> EAIKKLVGLQAKTAVVIRDGKEIAVPVE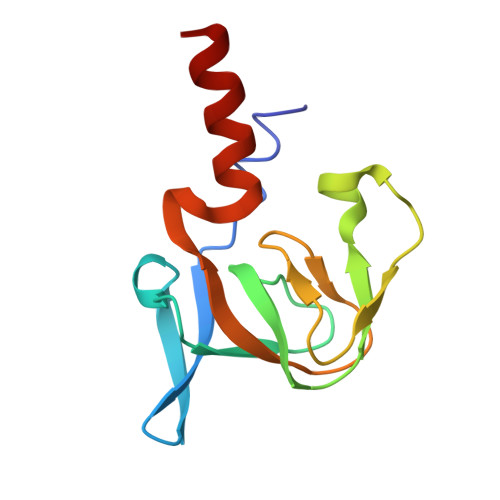EVAVGDIVIVRPGEKIPVDGVVVEGESYVDESMISGEPVPVLKSKGDEVFGATINNTGVLKIRATRVGGETLLAQIVKLVEDAMG> MAGHHHHHHGSAENLYFQGPISPIETVPVKLKPGMDGPKVKQWPLTEEKIKALVEICTEMEKEGKISKIGPENPYNTPVFAIKKKDSTKWRKLVDFRELNKRTQDFWEVQLGIPHPAGLKKKKSVTVLDVGDAYFSVPLDEDFRKYTAFTIPSINNETPGIRYQYNVLPQGWKGSPAIFQSSMTKILEPFRKQNPDIVIYQYMDDLYVGSDLEIGQHRTKIEELRQHLLRWGLTTPDKKHQKEPPFLWMGYELHPDKWTVQPIVLPEKDSWTVNDIQKLVGKLNWASQIYPGIKVRQLCKLLRGTKALTEVIPLTEEAELELAENREILKEPVHGVYYDPSKDLIAEIQKQGQGQWTYQIYQEPFKNLKTGKYARMRGAHTNDVKQLTEAVQKITTESIVIW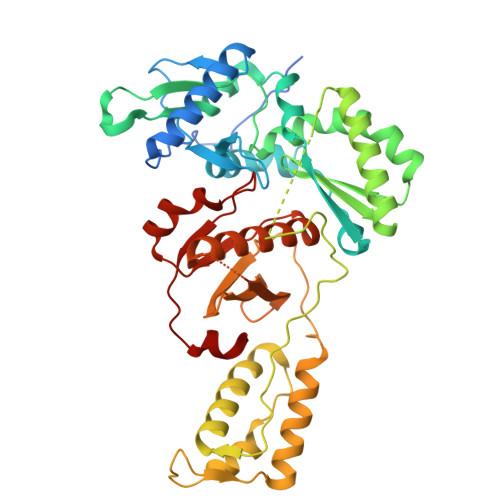GKTPKFKLPIQKETWETWWTEYWQATWIPEWEFVNTPPLVKLWYQ>[6x]SNAMDLTILHDCFDALQRAPTAEAAFPPIAAAAAALGFRY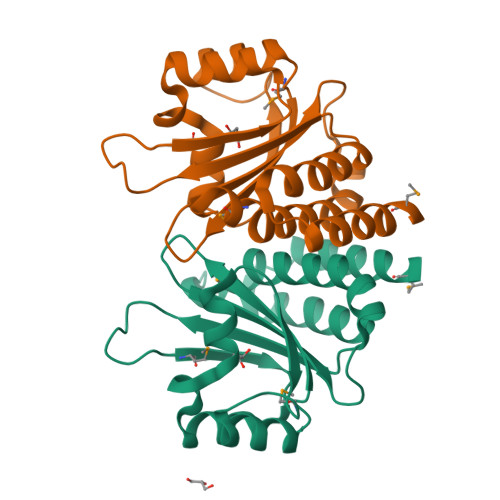CVYGLRRTLPLARPDMQIVGNHPREWEHRYVKFGYVTIDPIIKRVASQPRPVVWNAFDEPGDTAFWHDAACFGMRYGWSHGGYDRAGNLGVLTLVRDTTPLDADEISRLRAPCASLSHAAHAYLMPRLADPIA>SVYKVLLLGAPGVGKSA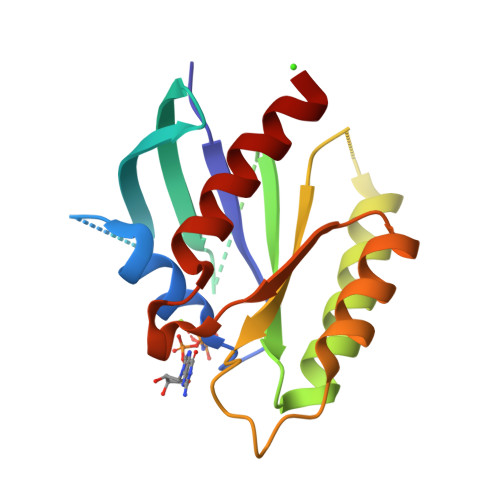LARIFGGVEDGPEAEAAGHTYDRSIVVDGEEASLMVYDIWEQDGGRWLPGHCMAMGDAYVIVYSVTDKGSFEKASELRVQLRRARQTDDVPIILVGNKSDLVRSREVSVDEGRACAVVFDCKFIETSAALHHNVQALFEGVVRQIRLRR[2x]>[4x]MGSSHHHHHHSSGENLYFQSHMSAPTMSTHLADHYNQAWLFAARAHRNQTLSGSPLPYL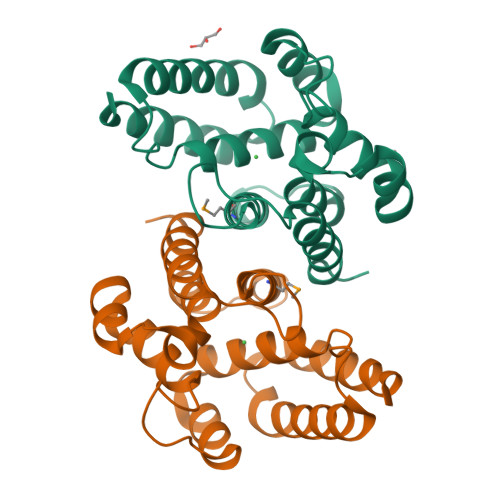VHLGMVANELLAADRDGAIERLGETLQIAVLHDTLEDTATSPEELRQQFGEFVCAGVQALSKRVGDGPKRSLDDYLQALAEGPAQYALVKLCDRITNLQPPPQTWNQDKIANYHQESQLILARLGHAHAATARRLREKIEHYRQYY>[2x]GIDPFTADKGKCGLPEIFDPPEELERKVWELARLVWQSSSVVFHTGAGISTASGIPDFRGPHGVWTMEERGLAPKFDTTFESARPTQTHMALVQLERVGLLRFLVSQNVDGLHVRSGFPRDKLAELHGNMFVEECAKCKTQYVRDTVVGTMGLKATGRLCTVAKARGLRACRGELRDTILDWEDSLPDRDLALADEASRNADLSITLGTSLQIRPSGNLPLATKRRGGRLVIVNLQPTKHDRHADLRIHGYVDEVMTRLMKHLGLEIPAWDGPRVLERALPPLPRPPTPKLEPKEESPTRIN

Sirtuins are NAD+-dependent protein lysine deacylases that sense the cellular nutrient status, regulate energy metabolism and stress responses, and have been implicated in aging processes and aging-related diseases. Sirtuins feature differing substrate acyl selectivities. Here, we analyse modulation of Sirt6 and other isoforms by quercetin and its derivatives in activity and binding assays and through crystal structure analyses of modulator complexes of Sirt6 and Sirt2. Our results hence reveal sites and mechanisms for Sirtuin modulation by quercetin derivatives and provide helpful insights for Sirt6 modulator development.

Catechin gallate (CG) is the most potent quercetin derivative reported to inhibit rather than activate Sirt6-dependent deacetylation (IC50 2.5 ± 0.1 μM). Testing CG in our MS assay confirmed the surprising inhibitory effect of this closely quercetin-related compound, albeit with slightly lower potency (IC50 80 ± 15 μM). To rationalize the inhibitory effect, we determined a crystal structure of a Sirt6/CG complex at 2.0 Å resolution. The bound inhibitor CG is well-defined by electron density and occupies the same binding region as the activator quercetin, with identical positions for their catechol moieties but a rotated chromen-4-one in GC to accommodate its additional, bulky trihydroxy benzoyl group. The chromen-4-one now interacts with Trp71 of the acyl channel exit, and the trihydroxy benzoyl group forms hydrophobic interactions with the other side of the exit funnel and a polar contact to the Gly155 backbone. The inhibitor does not overlap with the binding pocket for acetyl substrate but the catechol group assumes a position partly overlapping with the NAM moiety of the NAD+ cosubstrate. Testing CG inhibition at different NAD+ concentrations did not result in significant changes of residual activity, however, indicating that the inhibition is not based on NAD+ competition. The inhibitor CG differs from activators in a slight rotation of the catechol moiety, and more drastically in a tilted position of the chroman and the presence of its additional bulky substituent, orienting them toward N-terminus and Val154, respectively. The Val154/Gly155 peptide bond flips to provide space, but this and other differences in protein conformation are subtle. The bulky group pointing toward the N-terminus is CG’s dihydrochroman, and its strong tilt compared to quercetin/cyanidin is due to the saturated C-ring in CG.>[18x]TLIELMIVVAIIGILAAIAIPQYQNYIAKSQVSRVMSETGSLKTVIETCILDGKTAANCELGWTNSNLLG;>STAAVTGQTGLTITYPASATESAAIQGTFGNSAAIKIKNQTLTWTRTPEGAWSCATTVEAKFKPAGCAS[18x];> MNMYKWVPESIRDSGEGQPSYSNNGDYAPSGPWVAAGIHTMPQSLRDSMRNSIMVTAQARRDVIGPEWGPDGRFTGYASVIGTPDPKPADIVNKFTVERRPVSNGNFQQRVKAGDIVVAPYTSDGKITVKLVAGQKDISSTPDYDYRIDSSLASSAGFVVAGERWYYTKRHFIIPRYFQNWRMRRRKYVTGWVMPTFYSPKEIFNRLKDSLVPDTGLVTQVWADNNTKRMDFLTAMAEIPQTLSSFLDALGYLGSLIKDFKRRRFFLNKAHQRIRNKLGVSFAERRSQIVSKYDRKIA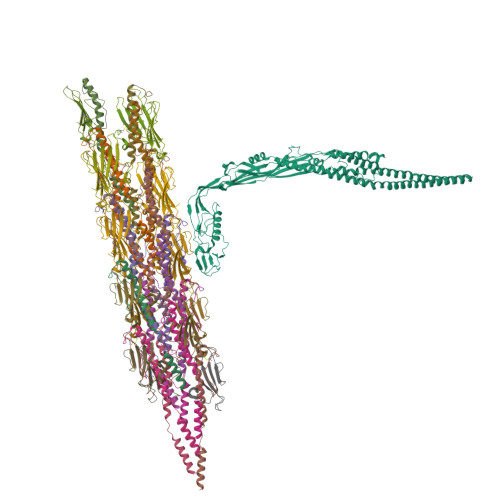SARKPAIIVKLRQRKEKALKALDKMRVREEKKMIREFATQAASLWLSFRYEIMPLYYQSQDVLDVIANSTSEFMTSRDFVAKAINIGIPLEWNLDQENLVSQPRHNVMVKSKLSPENNIGKTLSVNPFTTAWELLTLSFVVDWFVNFGDVIAGFTGGYSDDSGATASWRFDDKKVFHLKNIPSAMVIVDINFYTRQVIDPRLCGGLAFSPKLNLFRYLDAMSLSWNRSRLKISRAT>[12x]MPFITVGQENSTSIDLYYEDHGTGVPVVLIHGFPLSGHSWERQSAALLDAGYRVITYDRRGFGQSSQPTTGYDYDTFAADLNTVLETLDLQDAVLVGFSMGTGEVARYVSSYGTARIAAVAFLASLEPFLLKTDDNPDGAAPQEFFDGIVAAVKADRYAFYTGFFNDFYNLDENLGTRISEEAVRNSWNTAA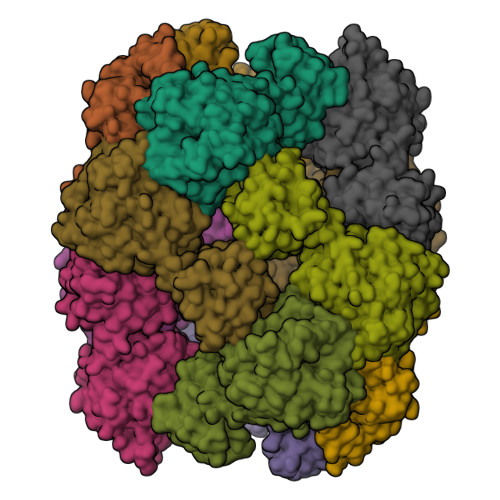SGGFFAAAAAPTTWYTDFRADIPRIDVPALILHGTGDRTLPIENTARVFHKALPSAEYVEVEGAPHGLLWTHAEEVNTALLAFLAKALEAQKQKLLTEVETYVLSIIPSGPLKAEIAQRLEDVFAGKNTDLEVLMEWLKTRPILSPLTKGILGFVFTLTVPSERGLQRRRFVQNALNGNGDPNNMDKAVKLYRKLKREITFHGAKEISLSYSAGALASCMGLIYNRMGAVTTEVAFGLVCATCEQIADSQHRSHRQLEHHHHHH> GPLGSELAYA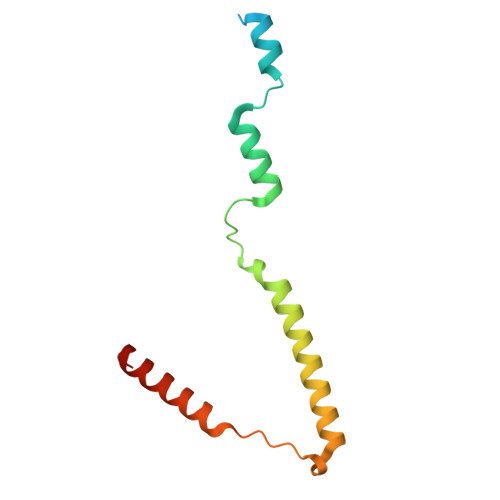LNNFDKQIIVDPLSFSEERFRPSLEERLESIISGAALMADSSCTRDDRRERIVAECNAVRQALQDLLSEYMGNAGRKERSDALNSAIDKMTKKTRDLRRQL>[4x]MFHSSAMVNSHRKPMFNIHRGFYCLTAILPQICICSQFSVPSSYHFTEDPGAFPVATNGERFPWQELRLPSVVIPLHYDLFVHPNLTSLDFVASEKIEVLVSNATQFIILHSKDLEITNATLQSEEDSRYMKPGKELKVLSYPAHEQIALLVPEKLTPHLKYYVAMDFQAKLGDGFEGFYKSTYRTLGGETRILAVTDFEPTQARMAFPCFDEPLFKANFSIKIRRESRHIALSNMPKVKTIELEGGLLEDHFETTVKMSTYLVAYIVCDFHSLSGFTSSGVKVSIYASPDKRNQTHYALQASLKLLDFYEKYFDIYYPLSKLDLIAIPDFAPGAMENWGLITYRETSLLFDPKTSSASDKLWVTRVIAHELAHQWFGNLVTMEWWNDIWLNEGFAKYMELIAVNATYPE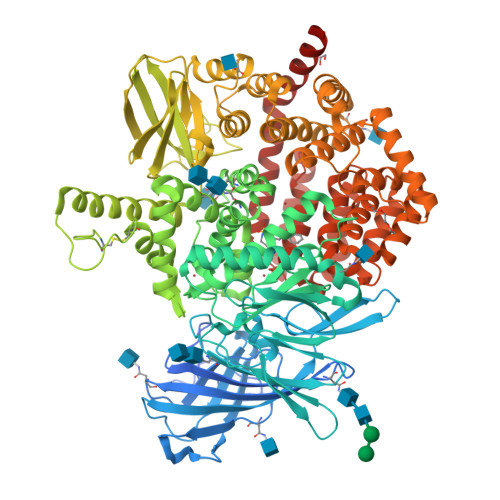LQFDDYFLNVCFEVITKDSLNSSRPISKPAETPTQIQEMFDEVSYNKGACILNMLKDFLGEEKFQKGIIQYLKKFSYRNAKNDDLWSSLSNSCLESDFTSGGVCHSDPKMTSNMLAFLGENAEVKEMMTTWTLQKGIPLLVVKQDGCSLRLQQERFLQGVFQEDPEWRALQERYLWHIPLTYSTSSSNVIHRHILKSKTDTLDLPEKTSWVKFNVDSNGYYIVHYEGHGWDQLITQLNQNHTLLRPKDRVGLIHDVFQLVGAGRLTLDKALDMTYYLQHETSSPALLEGLSYLESFYHMMDRRNISDISENLKRYLLQYFKPVIDRQSWSDKGSVWDRMLRSALLKLACDLNHAPCIQKAAELFSQWMESSGKLNIPTDVLKIVYSVGAQTTAGWNYLLEQYELSMSSAEQNKILYALSTSKHQEKLLKLIELGMEGKVIKTQNLAALLHAIARRPKGQQLAWDFVRENWTHLLKKFDLGSYDIRMIISGTTAHFSSKDKLQEVKLFFESLEAQGSHLDIFQTVLETITKNIKWLEKNLPTLRTWLMVNTRHHHHH>MRPGIRKLVVLNPRAYKGGSGHTTFYLLIPKDIAEALDIKPDDTFILNMEQKDG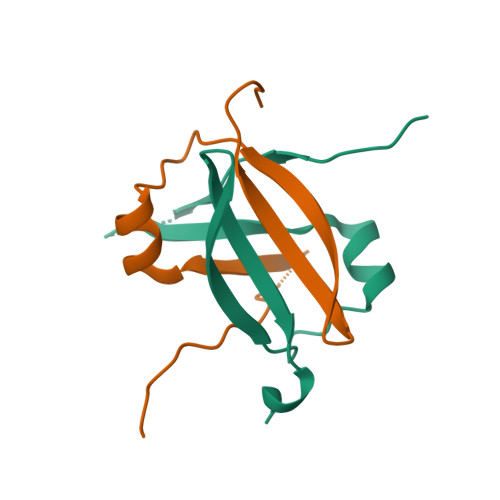DIVLSYKRVKELKI[2x]> MTQFTQNTAMPSSLWQYWRGLSGWNFYFLVKFGLLWAGYLNFHPLLNLVFAAFLLMPLPRYSLHRLRHWIALPIGFALFWHDTWLPGPESIMSQGSQVAGFSTDYLIDLVTRFINWQMIGAIFVLLVAWLFLSQWIRITVFVVAILLWLNVLTLAGPSFSLWPAGQPTTTVTTTGGNAAATVAATGGAPVVGDMPAQTAPPTTANLNAWLNNFYNAEAKRKSTFPSSLPADAQPFELLVINICSLSWSDIEAAGLMSHPLWSHFDIEFKNFNSATSYSGPAAIRLLRASCGQTSHTNLYQPANNDCYLFDNLSKLG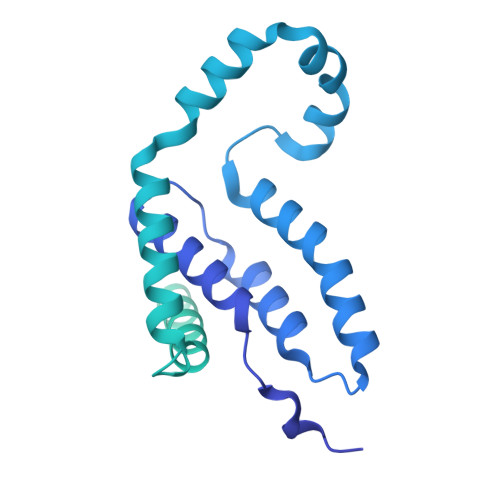FTQHLMMGHNGQFGGFLKEVRENGGMQSELMDQTNLPVILLGFDGSPVYDDTAVLNRWLDVTEKDKNSRSATFYNTLPLHDGNHYPGVSKTADYKARAQKFFDELDAFFTELEKSGRKVMVVVVPEHGGALKGDRMQVSGLRDIPSPSITDVPVGVKFFGMKAPHQGAPIVIEQPSSFLAISDLVVRVLDGKIFTEDNVDWKKLTSGLHKQHRSPRTQMQ> NEKLAKKKIVSIDAGRKYFSPEQLKEII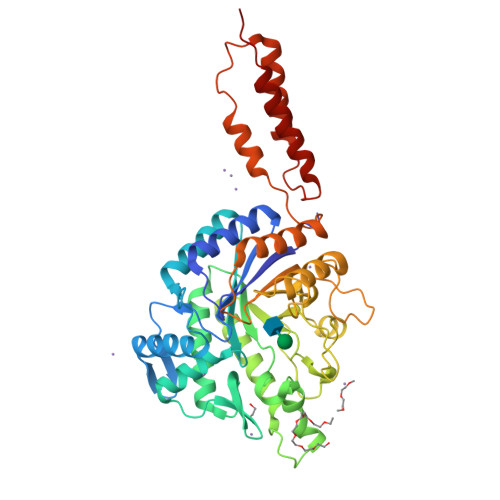DKAKHYGYTDLHLLVGNDGLRFMLDDMSITANGKTYASDDVKRAIEKGTNDYYNDPNGNHLTESQMTDLINYAKDKGIGLIPTVNSPGHMDAILNAMKELGIQNPNFSYFGKKSARTVDLDNEQAVAFTKALIDKYAAYFAKKTEIFNIGLDQYANDATDAKGWSVLQADKYYPNEGYPVKGYEKFIAYANDLARIVKSHGLKPMAFNDGIYYNSDTSFGSFDKDIIVSMWTGGWGGYDVASSKLLAEKGHQILNTNDAWYYVLGRNADGQGWYNLDQGLNGIKNTPITSVPKTEGADIPIIGGMVAAWADTPSARYSPSRLFKLMRHFANANAEYFAADYESAEQALNEVPKDLNRYTAESVTAVKEAEKAIRSLDSNLSRAQQDTIDQAIAKLQETVNNLTLTP> MADNLPSDFDVIVIGTGLPESIIAAACSRSGQRVLHVDSRSYYGGNWASFSFSGLLSWLKEYQENNDVVTENSMWQEQILENEEAIPLSSKDKTIQHVEVFCYASQDLHKDVEEAGALQKNHASVTSAQSAEAAEAAETSCLPTAVEPLSMGSCEIPAEQSQCPGPESSPEVNDAEATGKKENSDAKSSTEEPSENVPKVQDNTETPKKNRITYSQIIKEGRRFNIDLVSKLLYSRGLLIDLLIKSNVSRYAEFKNITRILAFREGTVEQVPCSRADVFNSKQLTMVEKRMLMKFLTFCVEYEEH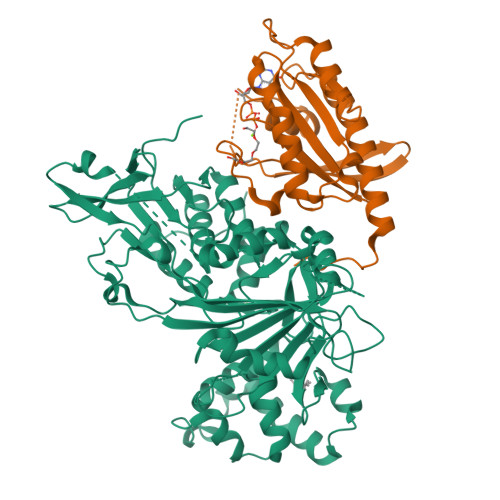PDEYRAYEGTTFSEYLKTQKLTPNLQYFVLHSIAMTSETTSCTVDGLKATKKFLQCLGRYGNTPFLFPLYGQGELPQCFCRMCAVFGGIYCLRHSVQCLVVDKESRKCKAVIDQFGQRIISKHFIIEDSYLSENTCSRVQYRQISRAVLITDGSVLRTDADQQVSILTVPAEEPGSFAVRVIELCSSTMTCMKGTYLVHLTCMSSKTAREDLERVVQKLFTPYTEIEAENEQVEKPRLLWALYFNMRDSSDISRDCYNDLPSNVYVCSGPDSGLGNDNAVKQAETLFQQICPNEDFCPAPPNPEDIVLDGDSSQQEVPESSVTPETNSETPKESTVLGNPEEPSE;> MTSRKKVLLKVIILGDSGVGKTSLMNQYVNKKFSNQYKATIGADFLTKEVMVDDRLVTMQIWDTAGQERFQSLGVAFYRGADCCVLVFDVTAPNTFKTLDSWRDEFLIQASPRDPENFPFVVLGNKIDLENRQVATKRAQAWCYSKNNIPYFETSAKEAINVEQAFQTIARNALKQETEVELYNEFPEPIKLDKNERAKASAESCSC> GPHMEEIMQSDSKIEKMLPDGGRLVVFPNGTRKELSADGQTVKVMFFNGDVKHTMPDQRVIYYYAEAQTTHITYPDGMEVLQFPNNQTVKHFPDGRKEITFPDQTVKTLHPDGREESVLTDGTIIQLNPDGSKVIQFNTGQREIHTADFKRREYPDGTVKTVYSDGRQETQYPTGRVRLKDPQGKVIMDTKA

Of particular interest in this regard is the putative centriolar CPAP–STIL complex, as mutations in both components result in MCPH. CPAP and STIL are strictly required for centriole assembly: STIL at a very early stage and CPAP slightly later, possibly by controlling the organisation and length of the centriolar microtubules. Instead, we demonstrate that the TCP domain of CPAP constitutes a novel proline-rich-motif (PRM) recognition-domain that specifically binds to a short target motif in STIL. Our mutational analysis of the interface demonstrates a remarkable correlation between the ability of mutant proteins to bind to one another in vitro and their ability to support centriole assembly in vivo, providing compelling support for our structural model of the metazoan CPAP–STIL complex. These data strongly suggest that the interaction between CPAP and STIL is a conserved, essential step in centriole biogenesis.

Intriguingly, a MCPH mutation (E1235V) in the conserved C-terminal domain of CPAP (the so-called TCP-domain or G-Box) appeared to weaken this yeast-two-hybrid interaction. The involvement of CPAP E1021 in the interaction with STIL in zebrafish is potentially significant, as the equivalent residue in human CPAP (E1235) is mutated to valine in some MCPH patients. To test whether this mutation disrupts the organisation of the TCP domain, we obtained the crystal structure of D. rerio CPAP937–1124 carrying the E1021V mutation. The structure of the wild-type and the mutant TCP domain were virtually identical (RMSD = 0.1 Å over 142 Cα pairs) demonstrating that the TCP domain structure was not compromised. ITC experiments with WT D. rerio STIL404–448 showed that the mutation of residues F978, Y994, and F1015 decreased the binding strength by ∼20 to 40-fold, while mutation of E1021 decreased the binding strength by approximately eightfold. Taken together these results lend strong support to our structural model and indicate that the E1021V MCPH mutation leads to roughly an order of magnitude decrease in affinity of the CPAP–STIL interaction. The structures we report here reveal that E1235 is one of the several residues involved in the binding interface with STIL, making an important sidechain–mainchain contact. This structural model explains how the E1235V mutation can compromise complex formation, and we have confirmed that this is the case with zebrafish proteins in vitro.(P-IODOPHENYLACETYLAMINO)METHYLPHOSPHINIC 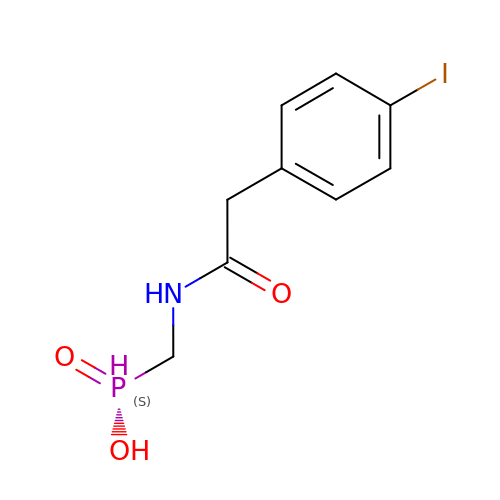ACID | C9 H11 I N O3 P | NJMHQBSYSLWOQF-UHFFFAOYSA-N>MGSSHHHHHHSSSAALEVLFQGP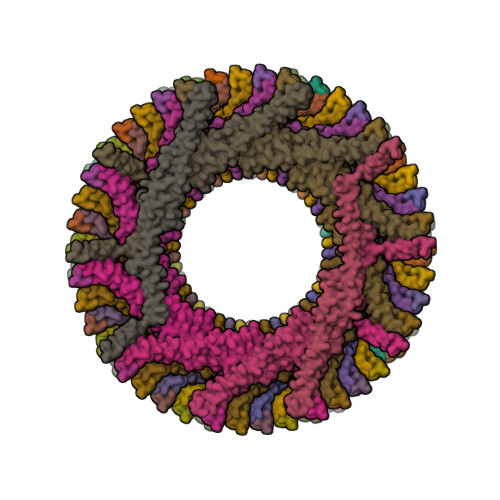MELFNRVGRVLKSQLTHWQQQQEAPEDLLERLLGEMELELIELRRALAQTIATFKSTERQRDAQQLIAQRWYEKAQAALDRGNEQLAREALGQRQSYQSHTEALGKSLGEQRALVEQVRGQLQKLERKYLELKSQKNLYLARLKSAIAAQKIEEIAGNLDNASASSLFERIETKILELEAERELLNPPPSPLDKKFEQWEEQQAVEATLAAMKARRSLPPPSS[60x]>MHRTSNGSHATGGNLPDVASHYPVAYEQTLDGTVGFVIDEMTPERATASVEVTDTLRQRWGLVHGGAYCALAEMLATEATVAVVHEKGMMAVGQSNHTSFFRPVKEGHVRAEAVRIHAGSTTWFWDV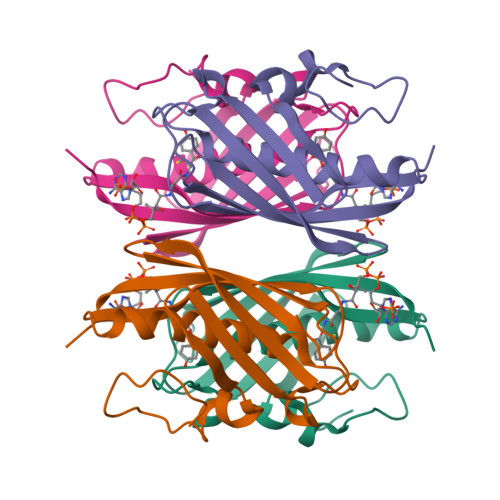SLRDDAGRLCAVSSMSIAVRPRRD[2x]>MGSSHHHHHHSSGLVPRGSSQQLTEREDIAIIGISGRYPQAENLQEFWKNLSEGTDCITEIPNDRWDHSLYYDADKDKEGKTYGKWGGFLKDVDKFDPQFFSISPRDAKLMDPQERLFLQCVYETMEDAGYTRKKLTEKSGDLLGANVGVYVGVMYEEYQLYGAEEQARGKSLALTGNPSSIANRASYVFGFNGPSMALDTMCSSSLTAIHLACQSLRNGECEAAFAGGVNVSVHPNKYLMLGQNRFLSSKGRCESFGEGGDGYVPGEGVGAVLLKPLSKAKADGDHIYGLIKGTAVNHDGKTNGYSVPNPNAQAAVIKQALKDAGTDPRAVSYI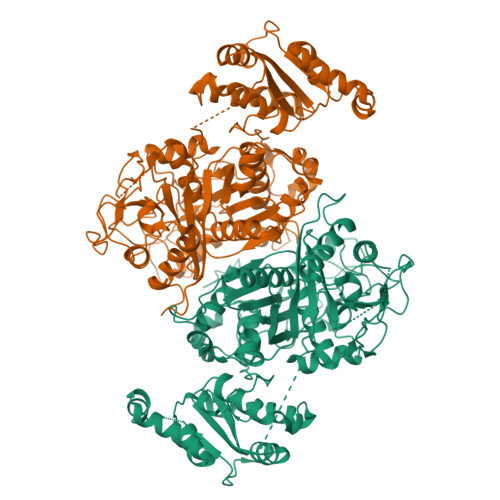EAHGTGTSLGDPIEITGLTKAFSEQTQDKQFCAIGSAKSNIGHCESAAGIAGLTKVLLQMKHKQLAPSLHSRTLNPNIDFLATPFKVQQTLEEWKRPVINENGVNKELPRTAGLSSFGAGGVNAHIVIEEYSADEDKETAFAAPHPSMIVLSAKNEQRLQKRAKRLLDALRSGRYREADLSRIAYTLQVGREPMEERLGMIVSNLRELEEKLDEFTGGKESIDQLYRGQVKQNKDTMALFTADEDMEKTIEAWLEKGKAAKVLELWVKGLPLNWDKLYQMGRPQKISLPAYPFAKDRYWIDTSAD[4x]Dual-specificity phosphatases (DUSPs) are a group of protein tyrosine phosphatases (PTPs) that can dephosphorylate both phosphoserine/threonine and phosphotyrosine. Despite their various substrate specificities, DUSPs exhibit a conserved catalytic mechanism mediated by a catalytic triad consisting of a Cys, an Arg, and an Asp in the active site and a phosphate-binding loop (PTP-loop) with a “HCxxGxxRS(T)” consensus motif. As an atypical DUSP family member, DUSP26 consists of an N-terminal domain (residues 1–60) as well as a conserved catalytic domain (DUSP26-C, residues 61–211). DUSP26 dephosphorylates pSer20 and pSer37 in the p53 transactivation domain (TAD) to inhibit the p53 tumor suppressor function and thereby results in the chemoresistance of neuroblastoma cells to doxorubicin-induced apoptosis.

In this study, we determined the crystal structure of a catalytically active form of DUSP26 with an N-terminal extension (residues 39–211, referred to as DUSP26-N) at 2.0 Å resolution. To gain insight into the structural basis for the catalytic activity of DUSP26, we determined the crystal structure of a catalytically active form of DUSP26, DUSP26-N. Because the active site cysteine of the phosphatase with a low pKa value is susceptible to oxidation, we mutated the active site cysteine (Cys152) to serine, which does not affect the structure or substrate binding, for crystallization. As shown in the structure of DUSP26-C, the DUSP26-N (C152S) monomer contains a central twisted five-stranded β-sheet (β1-β5) sandwiched by two α-helix bundles. Despite their close resemblance, the most noticeable difference between DUSP26-N (C152S) and DUSP26-C lies in the presence of an additional α1-helix in the N-terminus of DUSP26-N (C152S). By contrast, similar to VHR, the DUSP26-N (C152S) monomer adopts a “fold-back” conformation of the C-terminal α8-helix, which is packed against the catalytic core from the same subunit to form a four-helix bundle. Structural comparison with the catalytically active VHR and catalytically inactive DUSP26-C and MKP-4 showed that DUSP26-N (C152S) adopts a canonically active PTP-loop conformation, which is highly similar to that of VHR. Unlike those of DUSP26-C, which are flipped away from the active site, the backbone amide atoms of Val156 and Ser157 in the PTP loop of DUSP26-N (C152S) are pointed into the active site pocket. Together with the backbone amides of residues 153–154 and the guanidinium group of Arg158, they generate a positive electrostatic potential, which is crucial for the catalytic reaction of the cysteine thiolate anion. In the DUSP26-N (C152S) structure, the canonically active PTP-loop conformation is stabilized through formation of hydrogen bonds with the surrounding α7-α8 loop: Gly155-Arg186, Val156-Ile189, Val156-Pro190, and Ser157-Asn191.

>QHPFLNVFELERLLYTGKTACNHADEVWPGLYLGDQDMANNRRELRRLGITHVLNASHSRWRGTPEAYEGLGIRYLGVEAHDSPAFDMSIHFQTAADFIHRALSQPGGKILVHSAVGVSRSATLVLAYLMLYHHLTLVEAIKKVKDHRGIIPNRGFLRQLLALDRRLRQGLEALEHHHHHH[4x]> MTKDSGSGDDPVEVPAWPAHMERRRWPRDPTARKDRLAERSPALVPSRFSTRDLPPQEQFRSWRAHMAPLVD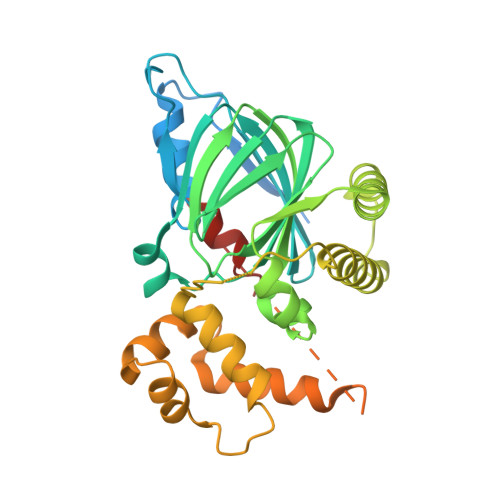VRLPDGVSEEDGFPAELTGWHLGDLLIVQQVTPAHSYERSQTMLRSSPIDHWNVGLFRSGRSWTEADRRVTETGPGEFFFRSLGYPYRGRMTDAASILLFMPYELLADDAGKLEGANNSVLSGNLADLLANYINGMEENLGNITVEEVPRIVRTIRDMVVACVAAVRPDAGGSQAKMGVMERAHRYIHLNLNSGDLTPETICRELGISRTRLYQLFEPSGGVLNYIRRRRLLQAYAELSDPTNNRPIGEIAEAAGFDLAANFTRAFSHEFGASPREIRKAAATERLATPVAPRERDRGATIGDWLKSVQG>KSSHTLKTANSYTDVTVSNSTKKAIRESNQYTDHKFHQLENRLDKLEKRL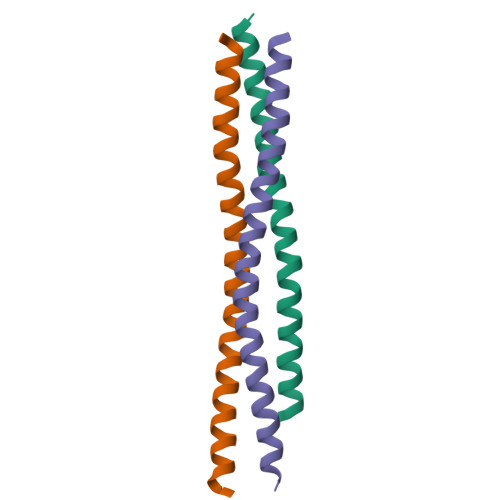LKLLASSAALNSLF[6x]>MGSSHHHHHHGSWTSAAVVTPPEPVQWQELEKTFTKLRVLDLDIKIDRTEAFNLFIKKFQSVSLLEEYLRSSPYVMDQLKEAKIDELDLHRAIVALSEKMKAVDDNASKKKDEPSLYTSWTLSFTAPTSEEAQTVLSGYIDYISALVVKESIENVRNKLEIKTQFEKEKLAQDRIKMKNQLDANIQRLNYSLDIANAAGIKKPVYSNGQAVKDDPDFSISLGADGIERKLEIEKAVTDVAELNGELRNRQYLVEQLTKANINDVNFTPFKYQL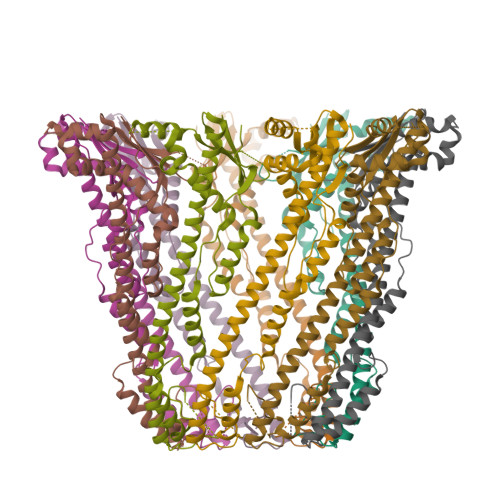SPSLPV[9x]> ARTKQTARXSTGGK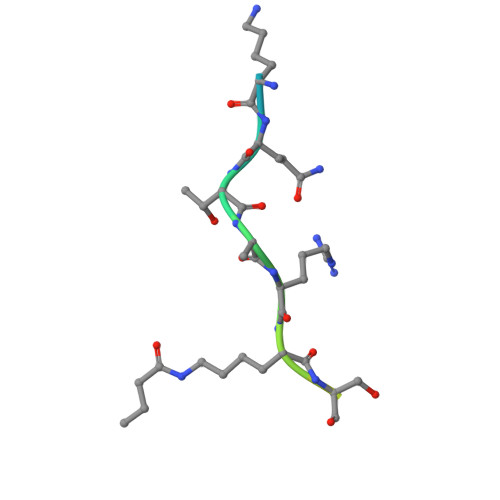APRKQ NSR is a member of the S41 protease family, specifically the C-terminal processing peptidases (CTPs). NSR from L. lactis TS1640 has been shown to degrade nisin by cleaving the peptide bond between MeLan28 in ring E and Ser29. In this study, we report the first structure of a nisin resistance protein, NSR from S. agalactiae COH1 (SaNSR). The present study reveals that the lanthionine ring E of nisin determines substrate specificity of the nisin resistance protein (NSR) and contributes to the coordination of the nisin cleavage site at the catalytic center.

We deleted this N-terminal transmembrane helix and included a His8-tag for purification purposes, resulting in soluble expression of SaNSR. SaNSR protein was crystallized and cubic crystals were obtained that diffracted up to 2.2 Å resolution. We solved the structure by Single Anomalous Dispersion (SAD) phasing, using crystals of selenomethionine-substituted protein (data and refinement statistics are shown in Table 1). The asymmetric unit contained four copies of SaNSR that were virtually identical (root mean square deviation (RMSD) between the monomers = 0.15–0.5 Å over 300 amino acids). A SaNSR monomer consists of eleven helices (α1-α11) and eleven β-strands (βa-βk), which form three domains: an N-terminal helical bundle and two protease subdomains. Altogether, these domains form a hydrophobic tunnel of ~10 Å width, which could very well harbor the nisin molecule. The protease core domain is formed by six strands βb-βg and five helices α5-α9. It contains the highly conserved TASSAEM region that harbors the previously identified catalytically active serine at position 23622 (Fig. 1, represented in blue). N-pep is predominantly bound to SaNSR via direct backbone interactions to amino acids 167NNTGGN172 of β-strand βd, which is part of the protease core domain and is structurally located on the opposite site of the TASSAEM sequence motif. The presence of N-pep within the tunnel is clearly an induced artifact of the crystallization procedure, since in the full-length SaNSR protein, another 30 amino acids are attached at the N-terminus of the N-pep sequence that form a transmembrane helix. Out of all residues of this helix, only the side chain of Asp110 is intruding into the tunnel, which neither forms an interaction to N-pep in the crystal structure nor in the NSRTail MD simulations. This suggests that the protease cap is not adopting a fully closed state, rather an intermediate state.

>[4x]MGSSHHHHHHHHSSGLVPRGSHLNIYLLPPSSERYGRVILDRVEQRGLYSQGRQWQIIRQRSEKKLKTSKSYQESRNIVQEAVRYGGGKHSQILSKETVRRDTLDSRYPEYRRLNEDILLITIPSISKLDKRSISHYSGKLQNILMEKSYKGLILDLSNNTGGNMIPMIGGLASILPNDTLFHYTDKYGNKKTITMKNIPLEALKISRKTINTKHVPIAIITNHKTASSAEMTFLSFKGLPNVKSFGQATAGYTTVNETFMLYDGARLALTTGIVSDRQGYKYENTPILPDQVTSLPLQESQSWLKSRINQN> MAVNSKYHHSCINCGGLNTDERNERGLPCEVCLPEDSPSDIYRALLERKTLKEYRFYHEFWNEYEDFRSFFKKKFGKDLTGYQRLWAKRIVQGKSFTMVAPTGVGKTTFGMMTALWLARKGKKSALVFPTVTLVKQTLERLQKLADEKVKIFGFYSSMKKEEKEKFEKSFEEDDYHILVFSTQFVSKNREKLSQKRFDFVFVDDVDAVLKASRNIDTLLMMVGIPEEIIRKAFSTIKQGKIYERPKNLKPGILVVSSATAKPRGIRPLLFRDLLNFTVGRLVSVARNITHVRISSRSKEKLVELLEIFRDGILIFAQTEEEGKELYEYLKRFKFNVGETWSEFEKNFEDFKVGKINILIGVQAYYGKLTRGVDLPERIKYVIFWGTPSMRFSLELDKAPRFVLARVLKEMGLIKAQENPDVEELRKIAKEHLTQKEFVEKVKEMFRGVVVKDEDLELIIPDVYTYIQASGRSSRILNGVLVKGVSVIFEEDEEIFESLKTRLLLIAEEEIIEEAEANWKELVHEVEESRRRSERELTDTSRSLLIIVESPTKAETLSRFLGRASSRKERNIIVHEAVTGEGVILFTATRGHVYDLVTKGGIHGVEEENGKFVPVYNSLKRCRDCGYQFTEDRDECPVCSSKNIDDKTETLRALREISLEADEILVATDPDVEGEKISWDVTQYLLPSTRSLRRIEMHEITRYGFKKARESVRFVDFNLVKAQIVRRVQDRWIGFELSGKLQKRFGRSNLSAGRVQSTVLGWIVEREEEYKKSEKDFTLLVLENGVNLEVEGKIADDVVTVVELQEAEEEKNPLPPYTTSSALSEISQKLRLGVQEVMDILQDLFEKGFITFHRTDSTRISLEGQNVARTYLRKIGKEDIFMGRSWSTEGAHEAIRPVKPIDARELEEMIEEGLIADLTKKHLRVYELIFNRFLASQSAAVKVKKQIVTVDVDGKRMGIEQIVEILRDGWNLFVPLTVSPRFEHRTYKIKEKKFYKKHTVPLFTQASIVEEMKKRGIGRPSTYAKIVEVLFRRGYVYEDKYKRVRPTRFGVMVYSYLKERYEKYVTEETTRRLEEIMDKVERGEEDYQATLRLLYEEIKSLMEEG

Reverse gyrase is a bacterial/archaeal type IA DNA topoisomerase that catalyzes the ATP-dependent introduction of positive supercoils into DNA. The general architecture of reverse gyrase has become evident from crystal structures of the enzymes from Archaeoglobus fulgidus and Thermotoga maritima. Both enzymes are large (>120 kDa) monomeric entities that consist of a helicase domain containing the ATP-binding site and a type IA topoisomerase domain fused on the same poly­peptide chain. The two parts of reverse gyrase, the helicase domain and the topoisomerase domain, are structurally connected by the latch, an insertion in the helicase subdomain H2. The latch couples the activity of the helicase domain to strand passage.

It contains the catalytic tyrosine residue that acts as a nucleophile for DNA cleavage. For the convenience of biochemical studies, this residue is often mutated to phenylalanine, which renders reverse gyrase inactive but still able to bind its substrates. The corresponding cleavage-deficient variant of reverse gyrase has also been used, but no information on the structural changes associated with this mutation is available. In parallel to the structure-determination efforts of T. maritima reverse gyrase with a minimal latch, we also determined the crystal structure of the rgyr_Y851F variant. The Tyr/Phe residue at position 851 stacks on Pro660 and is further encased by the side chains of Asp668, Phe844, His852 and Arg853. In all structures the guanidinium group of Arg853 remains fixed through a charged hydrogen bond to Asp670, but the aliphatic part of Arg853 can adopt slightly different rotamers. The α-helix is present in both wild-type structures but is in a slightly different conformation in the Y851F structure. In this study, we provide evidence that the cleavage-deficient Y851F variant of T. maritima reverse gyrase shares many structural characteristics with the wild-type enzyme.>MVRIYTLTLAPSLDSATI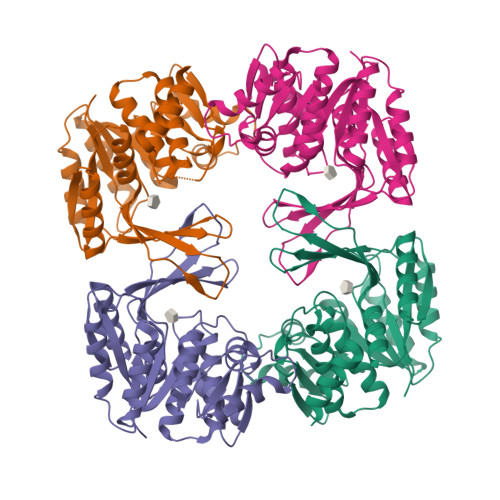TPQIYPEGKLRCTAPVFEPGGGGINVARAIAHLGGSATAIFPAGGATGEHLVSLLADENVPVATVEAKDWTRQNLHVHVEASGEQYRFVMPGAALNEDEFRQLEEQVLEIESGAILVISGSLPPGVKLEKLTQLISAAQKQGIRCIVDSSGEALSAALAIGNIELVKPNQKELSALVNRELTQPDDVRKAAQEIVNSGKAKRVVVSLGPQGALGVDSENCIQVVPPPVKSQSTVGAGDSMVGAMTLKLAENASLEEMVRFGVAAGSAATLNQGTRLCSHDDTQKIYAYLSR[4x]Members of the myomesin protein family function as molecular bridges that connect major filament systems in the central M-band of muscle sarcomeres, which is a central locus of passive stress sensing. To unravel the mechanism of molecular elasticity in such filament-connecting proteins, we have determined the overall architecture of the complete C-terminal immunoglobulin domain array of myomesin by X-ray crystallography, electron microscopy, solution X-ray scattering, and atomic force microscopy. Our data reveal a dimeric tail-to-tail filament structure of about 360 Å in length, which is folded into an irregular superhelical coil arrangement of almost identical α-helix/domain modules. The myomesin filament can be stretched to about 2.5-fold its original length by reversible unfolding of these linkers, a mechanism that to our knowledge has not been observed previously.

First, we determined the overall architecture of the complete myomesin domain array, including Ig domains My9–My10–My11–My12–My13, from crystal structures of a total of three filament fragments: the My9–My11 triplet, determined at 2.5 Å resolution; the My10–My11 doublet, at 1.9 Å resolution; and the homodimeric My11–My13 triplet at 3.5 Å resolution. Although the structure-based sequence similarity of the five Ig domains is generally below 25%, all Ig domains except My13 belong to different sub-classes of the C-set type Ig domain topology. Remarkably, all five Ig domains of the myomesin filament are connected by α-helices that are identical in terms of orientation with respect to the preceding Ig domain, and they form a substantial, structurally highly conserved Ig domain/helix interface with an area of 350–600 Å2. These interfaces involve loops that form the C-terminal tip region in each Ig domain, and residues from the first three helical turns form various specific interactions that shield the N-terminal part of each α-helix from being completely exposed. We refer hereafter to this as the “IgH” segment, which to our knowledge has not been found in any other muscle filament protein with repetitive Ig or Fn-III domains. Whereas long six-turn helices are found in the My10–My11 and My12–My13 connecting segments, the corresponding helices in the other two connecting segments, My9–My10 and My11–My12, are slightly shorter, with about four turns each. Because of the smaller length of their linkers, My9–My10 and My11–My12 show limited direct interactions in their respective Ig doublets, whereas in the other two doublets, My10–My11 and My12–My13, the neighboring My domains are too far away from each other to form an interface. The right-handed superhelix is defined by almost constant twist angles of neighboring My domains of 26–27°, except the arrangement of My12–My13, which has an average twist angle of 68° and thus appears to be less regular than preceding parts My9–My10–My11–My12 of the filament.

> GIDPFTKEVVVNVDDDGVISLNFECDKMTPKSEFSWSKDYVSTEDSPRLEVESKGNKTKMTFKDLGMDDLGIYSCDVTDTDGIASSYLIDEEELKRLLALSHEHKFPTVPVKSELAVEILEKGQVRFWMQAEKLSGNAKVNYIFNEKEIFEGPKYKMHIDRNTGIIEMFMEKLQDEDEGTYTFQLQDGKATNHSTVVLVGDVFKKLQKEAEFQRQEWIRKQGPHFVEYLSWEVTGECNVLLKCKVANIKKETHIVWYKDEREISVDEKHDFKDGICTLLITEFSKKDAGIYEVILKDDRGKDKSRLKLVDEA Dimethylsulfoniopropionate (DMSP) is a ubiquitous organosulfur compound in marine environments with important functions in both microorganisms and global biogeochemical carbon and sulfur cycling. Here, through comparative genomics analyses, genetic manipulations, and biochemical analyses, we identified an ABC (ATP-binding cassette)-type DMSP-specific transporter, DmpXWV, in Ruegeria pomeroyi DSS-3, a model strain of the MRG. DmpX, the substrate binding protein of DmpXWV, had high specificity and binding affinity towards DMSP. In Gram-negative bacteria, they usually consist of three subunits: a periplasmic substrate-binding protein (SBP) responsible for the primary recognition and binding of substrate, a transmembrane domain constituting the translocation pathway, and a cytoplasmic ATP-binding domain to hydrolyse ATP and provide energy for transport.

While DmpX proteins of R. pomeroyi DSS-3 and Pelagibacter sp. HTCC7211 did not yield crystals, a DmpX homologue from MRG strain Roseovarius nubinhibens ISM, RnDmpX, sharing 58% amino acid identity with R. pomeroyi DSS-3 DmpX, yielded good quality crystals when co-crystallization with DMSP was conducted. The recombinant RnDmpX also presented a high binding affinity for DMSP, with a Kd of 474 nM, and the crystal structure of RnDmpX in complex with DMSP was solved. RnDmpX comprises two domains connected by two hinge regions (Val106-Gly111 and Arg244-Val247), with a DMSP molecule bound between the two domains. The binding pocket of RnDmpX is composed of Trp35, Thr64 and Trp84 from domain I, and Glu113, Trp152, Ala153, Tyr200 and Trp202 from domain II. Residues Thr64 and Ala153 participate in binding DMSP through hydrogen bonds with the carboxyl group of DMSP. Glu113 also participates in binding DMSP through a water-mediated hydrogen bond with DMSP. The side chains of the four tryptophan residues form a hydrophobic cage to accommodate the tertiary sulfonium group of DMSP. In particular, we found that Tyr200 could form a hydrogen bond with the positive-charged sulfur of DMSP. When Tyr200 was mutated to Ala or Phe, the binding affinities of RnDmpX for DMSP were abolished, suggesting that this interaction plays an important role in DMSP binding. Thus, the hydrogen bond formed between Tyr200 and DMSP may represent a novel substrate binding and recognition pattern of SBPs.

> MTKINLATLSVIGFLGSASIAQAECGEVSITEMNWASASVVTTVATFLMEQGYGCAVTVVPSSTVPAVTSVSETGEPDILTELWLSSLPNYAKLEAQGTVRTLTEVLSDGGQEGWWVPQYLAEAHPEVTTIEGILANPDLVGGRFHRSPDGWAAAIVDSSLAKAWDLEGNGIEVFAHGSGETLATSIAAAYADREPWFGYYWAPTSVLGKFPMVMVDLGEFDADIHACNSKADCANVGKSPYPRARVITAVTPGFAEENPEIIEMLSNLSFTNDQMGAILAWQEENGASSEEAAVWFLSNNSDIWAGWVNDAARENLAALIP>[2x]PPYTVVYFPVRGRCAALRMLLADQ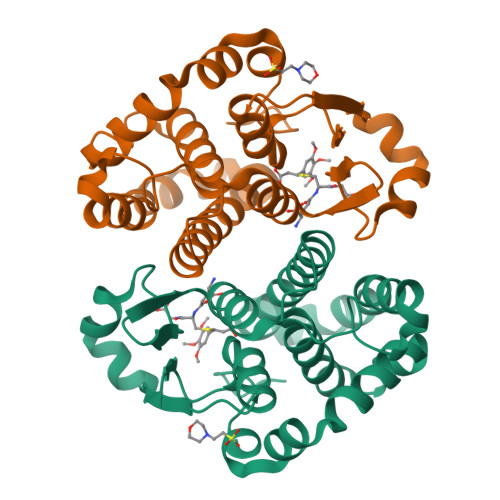GQSWKEEVVTVETWQEGSLKASCLYGQLPKFQDGDLTLYQSNTILRHLGRTLGLYGKDQQEAALVDMVNDGVEDLRCKYISLIYTNYEAGKDDYVKALPGQLKPFETLLSQNQGGKTFIVGDQISFADYNLLDLLLIHEVLAPGCLDAFPLLSAYVGRLSARPKLKAFLASPEYVNLPINGNGKQ> DYADNDSILLKHGWCEMLKGGVIMDVKNVEQAKIAEKAGAIGVMILENIPSELRNTDGVARSVDPLKIEEIRKC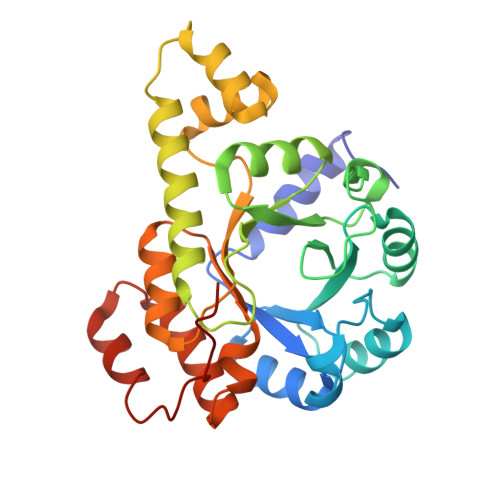ISINVLAKVRIGHFVEAQILEELKVDMLDESEVLTMADEYNHINKHKFKTPFVCGCTNLGEALRRISEGASMIRTKGEAGTGNIIEAIKHIRTVNNEIKYLCSLDESEVYNFAKKLRAPIDLILLTRKLKRLPVVNFAAGGIATPADAAMCMQLGMDGVFVGSGIFESENPQKMASSIVMAVSNFNNPKILLNVSLGLGKAMHGNTAA> MYYLGKELQKRSEELSRGFYELVYPPVDMYEEGGYLVVVADLAGFNKEKIKARVSGQNELIIEAEREITEPGVKYLTQ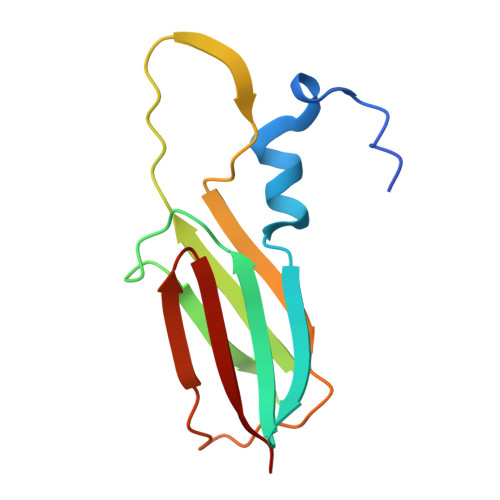RPKYVRKVIRLPYNVAKDAEISGKYENGVLTIRIPIA>GSRQELQPWQRATYDFFMPQNLREDLQKKQFATLQVIPNSGLPQLEHWHSLVPLDTSNRKNTSCFGYPSWVYKAQNSRNGRHYALRRLEGYRLTNEKAILNVMKDWKKIKNASIVTIHEVFTTREFGDSSLIFAYDFHPLSKTLQEHHFQPIHGNRYRPPPAVPENTIWGYICQIANALKTIHSNRLAARCLEPSKIILTDINRIRLSACAILDVVQFGMNSRSVVELQQEDFVKFGKLILSLATGTLPAHLNNIPAALETLGNKYSANLKSAVNWLLDTSSGETKTIEHFMTGIASQMTTFFDLALQDNDEKLFHLAREVENGRIARSLMKLLTILERGDYDGVPSWSETGDRYQLKLFRDYVFHRVDADGKPNLSIGHMLTCMSKLEAGVDENILLTSRDNETVFVLSYRELRQMYDRAFNELVKASKTGAPGANT[8x]

Two conserved complexes carry out the majority of deadenylation in the cytoplasm: Pan2–Pan3 and Ccr4–Not. As illustrated in Fig1A, Pan3 contains a zinc finger at its N-terminus, a pseudokinase domain (PK), a coiled coil and a highly conserved C-terminal domain (CTD) (Brown et al, 1996; Christie et al, 2013; Wolf & Passmore, 2014). Pan2 contains three functional domains: an N-terminal WD40 domain, an inactive ubiquitin C-terminal hydrolase (UCH) domain and a C-terminal exonuclease (Fig1A) (Boeck et al, 1996; Wolf & Passmore, 2014). In conclusion, through combined biochemical and structural approaches, we have shown that Pan3 is required to couple RNA binding to the Pan2 exonuclease activity.

We obtained crystals of Se-Met-labeled ctPan3 PKC (residues 205–640) with P1 symmetry and four Pan3 homodimers in the asymmetric unit that were solved using single-wavelength anomalous dispersion (SAD) methods. The ctPan3 structure consists of an N-terminal pseudokinase domain (residues 242–497) to which MgATP is bound, a central asymmetric coiled-coil domain (residues 499–538) and a C-terminal domain (residues 555–640) (Fig5C). Although ATP was bound to both pseudokinase domains, ATP was not added to crystallization conditions and is present in all copies in the asymmetric unit of the crystal. The pseudokinase lacks almost all catalytic residues and is predicted to be inactive (Christie et al, 2013). Two distinctive beta-hairpin ‘ears’ protrude from each C-terminal domain. A kink is formed in the coiled-coil region as a result of one of the CTDs (chain B) interacting with the pseudokinase from the other chain, introducing asymmetry into the Pan3 dimer. The pseudokinase and CTD domains of C. thermophilum Pan3 are similar to the recently reported structures for Drosophila (RMSDs of 1.13 Å and 0.87 Å, respectively) and Neurospora (RMSDs of 1.24 Å and 0.93 Å, respectively) proteins (Christie et al, 2013), indicating high structural conservation of Pan3. The principal difference between these structures is that the kink in the coiled coil of ctPan3 is more pronounced, resulting in twists of approximately 28° and 31°, respectively, of the CTD relative to the pseudokinase domain. Second, the highly conserved Pan3 pseudokinase/C-terminal domain also binds RNA but in a manner that is not specific for polyA (Fig4). This region has a theoretical pI of approximately 8.8, and examination of the surface potential reveals a substantial positive charge that could mediate electrostatic interactions with negatively charged RNA backbone phosphates.>MSLKIRDAYTIVTCPGRNFVTLKIVTESGTHGIGDATLNGREMAVAAYLDEHVVPALIGRDAGRIEDTWQYLYRGAYWRRGPVTMTAIAAVDMALWDIKAKAAGMPLYQLLGGKSRERVMTYAHCTGQTIEDCLGEVARHVELGYRAVRVQSGVPGIETTYGVAKTPGERYEPADSSLPAEHVWSTEKYLNHAPKLFAAVRERFGDDLHVLHDVHHRLTPIEAARLGKAVEPYHLFWLEDCVPAENQESLRLIREHTTTPLAIGEVFNSIHDCRELIQNQWIDYIRMPLTHGGGITAMRRVADLASLYHVRTGFHGPTDLSPVCLGAAIHFDTWVPNF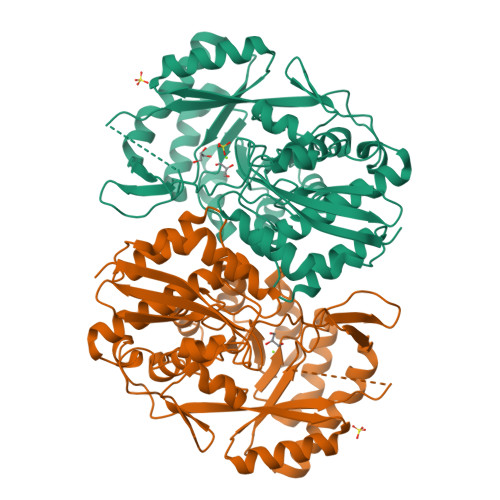GIQEHMPHTDETDAVFPHDYRFEDGHFLAGESPGHGVDIDEELAAKYPYERASLPVNRLEDGTLWHW[8x]> IDTLQLDNFLTTGFLDIIPLSQPLEFRREGLQHGVLDKLRSGKYPQQASLNLLRQPVEECRKMVFSFIQQALADGLRNVLIIH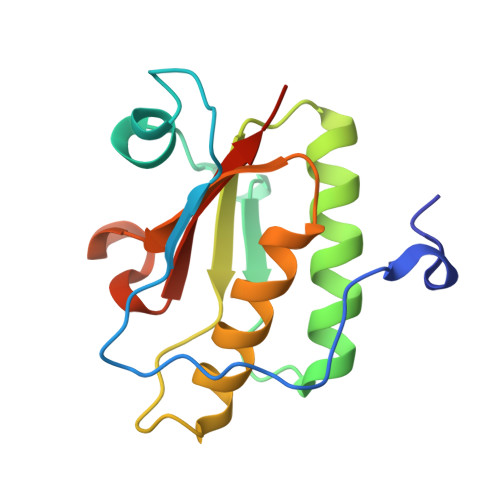GKGRDDKSHANIVRSYVARWLTEFDDVQAYCTALPHHGGSGACYVALRKTAQAK(3R)-1-[(4-chlorophenyl)methyl]pyrrolidin-3-ol | C11 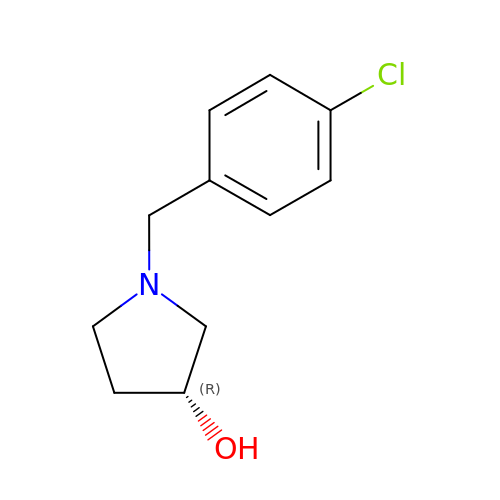H14 Cl N O | NVBPYTSZAGPUJC-LLVKDONJSA-N>MMTDKLNLNVLDAAFYSLEQTVVQISDRNWFDMQPSIVQDTLIAGAIQKFEFVYELSLKMMKRQLQQDAINTDDIGAYGFKDILREALRFGLIGDMSKWVAYRDMRNITSHTYDQEKAMAVYAQIDDFLIESSFLLEQLRQRNQY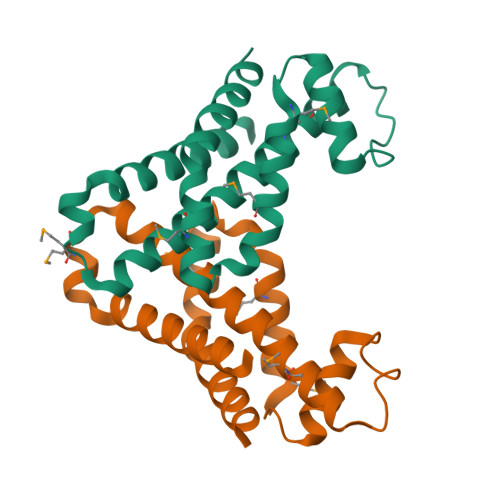D[4x]> GSMGKLSEQLKHCNGILKELLSKKHAAYAWPFYKPVDASALGLHDYHDIIKH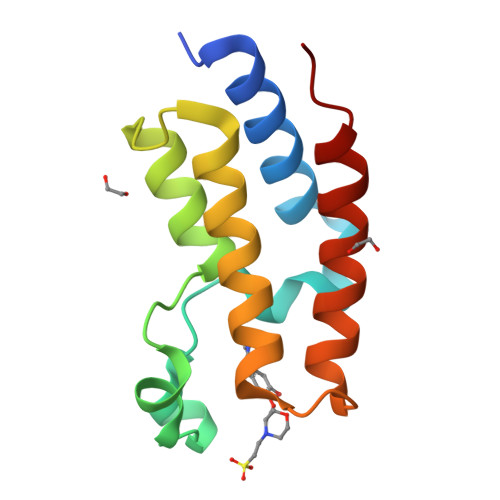PMDLSTVKRKMENRDYRDAQEFAADVRLMFSNCYKYNPPDHDVVAMARKLQDVFEFRYAKMPD>[2x]EYGDLHLFGPNQRPAPCY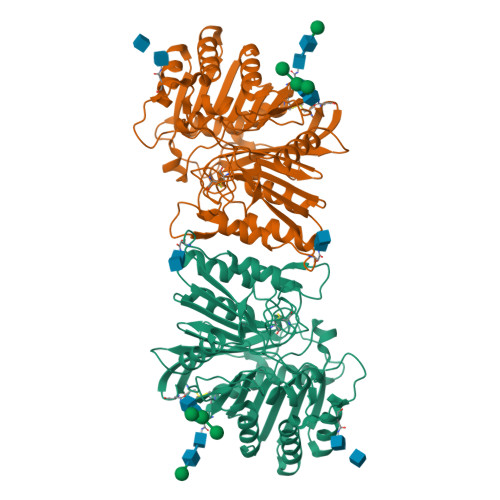DPCEAVLVESIPEGLDFPNASTGNPSTSQAWLGLLAGAHSSLDIASFYWTLTNNDTHTQEPSAQQGEEVLRQLQTLAPKGVNVRIAVSKPSGPQPQADLQALLQSGAQVRMVDMQKLTHGVLHTKFWVVDQTHFYLGSANMDWRSLTQVKELGVVMYNCSCLARDLTKIFEAYWFLGQAGSSIPSTWPRFYDTRYNQETPMEICLNGTPALAYLASAPPPLCPSGRTPDLKALLNVVDNARSFIYVAVMNYLPTLEFSHPHRFWPAIDDGLRRATYERGVKVRLLISCWGHSEPSMRAFLLSLAALRDNHTHSDIQVKLFVVPADEAQARIPYARVNHNKYMVTERATYIGTSNWSGNYFTETAGTSLLVTQNGRGGLRSQLEAIFLRDWDSPYSHDLDTSADSVGNACRLLLEVLFQ2-((5-(3,7-Diazabicyclo[3.3.1]nonan-3-yl)pyridin-3-yl)oxy)-N,N-dimethylethanamine 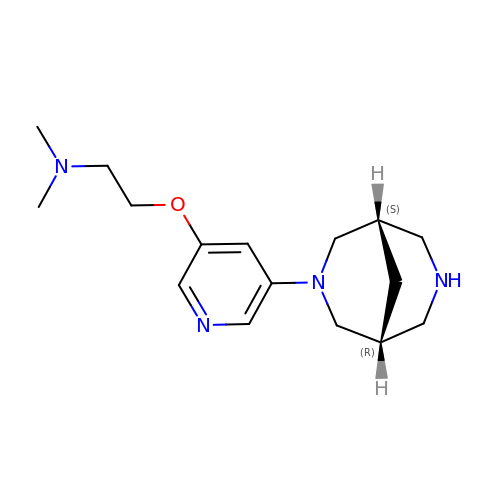| C16 H26 N4 O | YXMGPQOPWMCEQM-OKILXGFUSA-N> GAMGSPQEDSDIAFLIDGSGSIIPHDFRRMKEFVS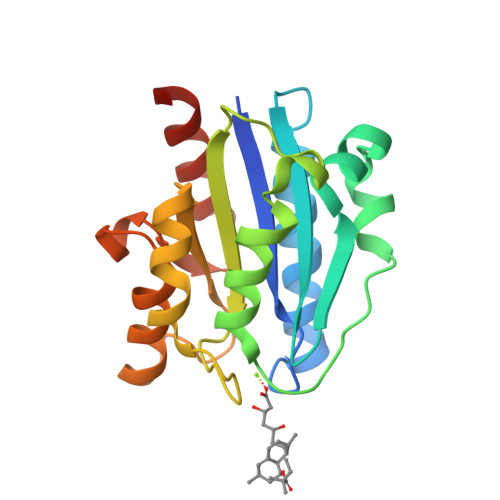TVMEQLKKSKTLFSLMQYSEEFRIHFTFKEFQNNPNPRSLVKPITQLLGRTHTATGIRKVVRELFNITNGARKNAFKILVVITDGEKFGDPLGYEDVIPEADREGVIRYVIGVGDAFRSEKSRQELNTIASKPPRDHVFQVNNFEALKTIQNQLREKGFAIEG>[6x]MTATVLLEVPFSARGDRIPDAVAELRTREPIRKVRTITGAEAWLVSSYALCTQVLEDRRFSMKETAAAGAPRLNALTVPPEVVNNMGNIADAGLRKAVMKAITPKAPGLEQFLRDTANSLLDNLITEGAPADLRNDFADPLATALHCKVLGIPQEDGPKLFRSLSIAFMSSADPIPAAKINWDRDIEYMAGILENPNITTGL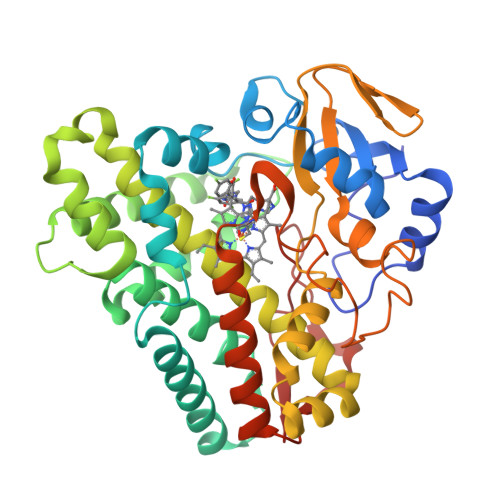MGELSRLRKDPAYSHVSDELFATIGVTFFGAGVISTGSFLTTALISLIQRPQLRNLLHEKPELIPAGVEELLRINLSFADGLPRLATADIQVGDVLVRKGELVLVLLEGANFDPEHFPNPGSIELDRPNPTSHLAFGRGQHFCPGSALGRRHAQIGIEALLKKMPGVDLAVPIDQLVWRTRFQRRIPERLPVLW2-AMINOTHIAZOLE 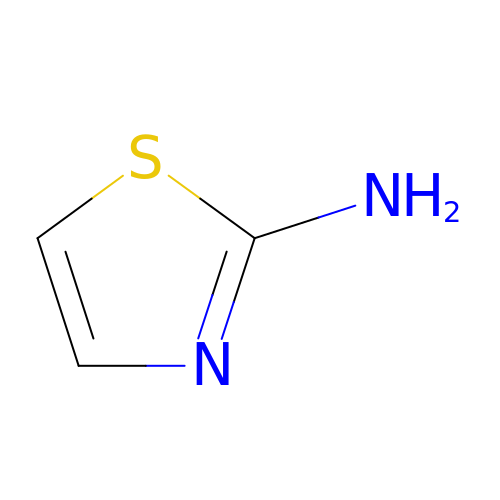| C3 H4 N2 S | RAIPHJJURHTUIC-UHFFFAOYSA-N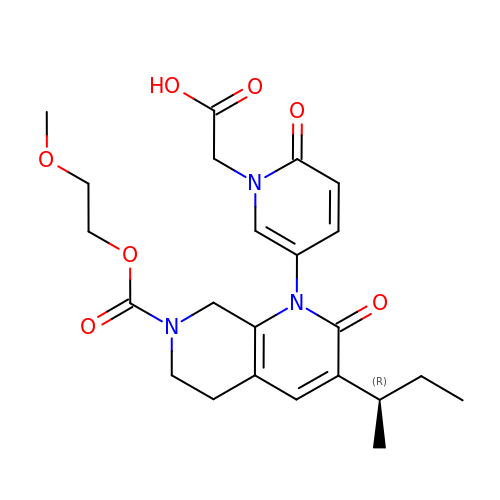[(5P)-5-{3-[(2R)-butan-2-yl]-7-[(2-methoxyethoxy)carbonyl]-2-oxo-5,6,7,8-tetrahydro-1,7-naphthyridin-1(2H)-yl}-2-oxopyridin-1(2H)-yl]acetic acid | C23 H29 N3 O7 | XFTKAVIYFGOXSI-OAHLLOKOSA-N> ATGDEWWAKCKQVDVLDSEMSYYDSDPGKHKNTVIFLHGNPTSSYLWRNVIPHVEPLARCLAPDLIGMGKSGKLPNHSYRFVDHYRYLSAWFDSVNLPEKVTIVCHDWGSGLGFHWCNEHRDRVKGIVHMESVVDVIESWDEWPDIEEDIALIKSEAGEEMVLKKNFFIERLLPSSIMRKLSEEEMDAYREPFVEPGESRRPTLTWPREIPIKGDGPEDVIEIVKSYNKWLSTSKDIPKLFINADPGFFSNAIKKVTKNWPNQ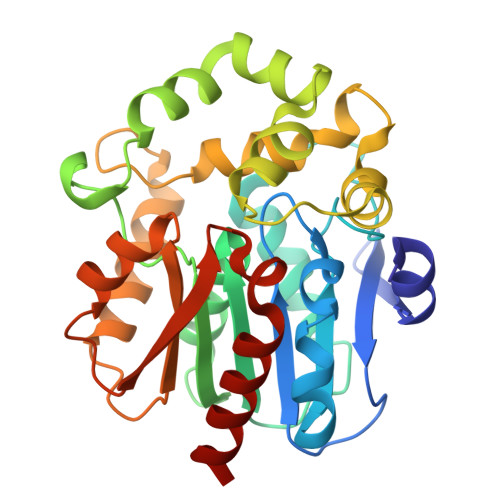KTVTVKGLHFLQEDSPEEIGEAIADFLNELT>MPTAKPEIVITYCTQCQWLLRAAWLAQELLSTFADDLGKVCLEPGTGGVFRITCDGVQVWERKADGGFPEAKALKQRVRDRIDPQRDLGHNDRP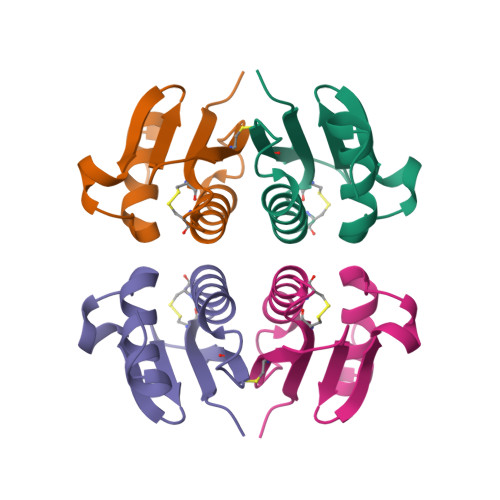SRLEHHHHHH[4x]>[2x]GHMAGASHDIHPPKVEYFDLRDHTNTDPKGFVRHVDHYRVEPWGLYMARTSDHPQFHYLESWLLPDLGLRASIFHYHPYH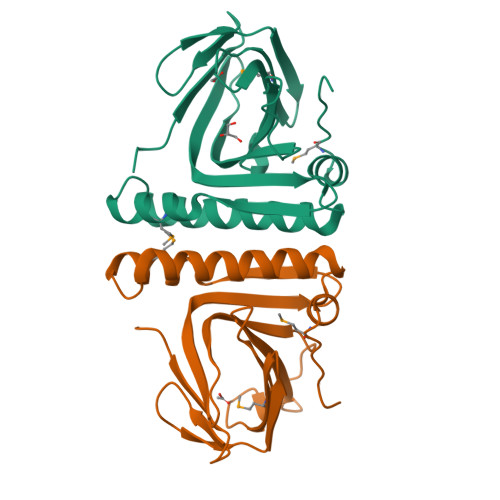QRDQDHYVDIGTFTRGDDVWKSEDHYLDLVVRTGRDTELLDVDELMEAHTTGLLDTATAEQAILTATTAIDGIAAHGHDLGRWLASIGMPIDWRGS>SLANTYLLQDHNTLTPYTPFTTPLNGGLDVVRAAHLHPSYELVDWKRVGDTKLVALVRSALVRVKFQDTTSSDQSNTNQNALSFDTQESQKALNGSQSGSSDTSGSNSQDFASYVLIFKAAPRATWVFERKIKLALPYVKQESQGSGDQGSNGKGSLYKTLQDLLVEQPVTPYTPNAGLARVNGVAQDTVHFGSGQESSWNSQRSQKGLKNNPGPKAVTGFKLDKGRAYRKLNESWPVYEPLDSTKEGKGKDESSWKNSEKTTAENDAPLVGMVGSGAAGSASSLQGNGSNSSGLKSLLRSAPVSVPPSSTSNQTLSLSNPAPVGPQAVVSQPAGGATAAVSVNRTASDTATFSKYLNTAQALHQMGVIVPGLEKWGGNNGTGVVASRQDATSTNLPHAAGASQTGLGTGSPREPALTATSQRAVTVVAGPLRAGNSSETDALPNVITQLYHTSTAQLAYLNGQIVVMGSDRVPSLWYWVVGEDQESGKATWWAKTELNWGTDKQKQFVENQLGFKDDSNSDSKNSNLKAQGLTQPAYLIAGLDVVADHLVFAAFKAGAVGYDMTTDSSASTYNQALAWSTTAGLDSDGGYKALVENTAGLNGPINGLFTLLDTFAYVTPVSGMKGGSQNNEEVQTTYPVKSDQKATAKIASLINASPLN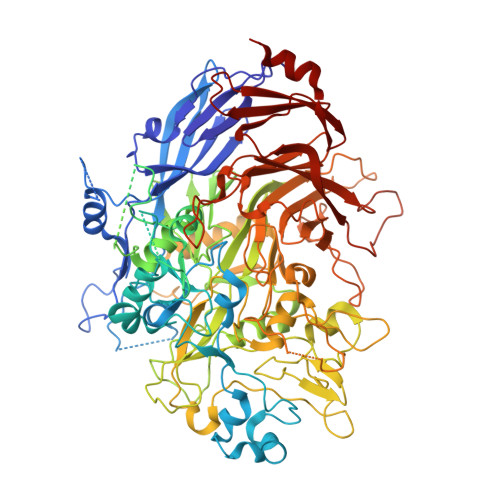SYGDDGVTVFDALGLNFNFKLNEERLPSRTDQLLVYGIVNESELKSARENAQSTSDDNSNTKVKWTNTASHYLPVPYYYSANFPEAGNRRRAEQRNGVKISTLESQATDGFANSLLNFGTGLKAGVDPAPVARGHKPNYSAVLLVRGGVVRLNFNPDTDKLLDSTDKNSEPISFSYTPFGSAESAVDLTTLKDVTYIAESGLWFYTFDNGEKPTYDGKQQQVKNRKGYAVITVSRTGIEFNEDANTTTLSQAPAALAVQNGIASSQDDLTGILPLSDEFSAVITKDQTWTGKVDIYKNTNGLFEKDDQLSENVKRR[2x]1-(5-TERT-BUTYL-1,3,4-OXADIAZOL-2-YL)-2-(METHYLAMINO)ETHANONE | C9 H15 N3 O2 | 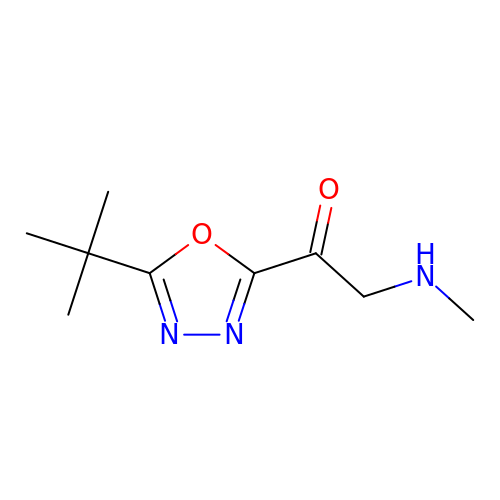CLBJJWUUSJAAPJ-UHFFFAOYSA-N> GSHMMSNANPYENNNPYAENYEMQEDLNNAPTGHYEGSDDFVAFMNKINSINANLSRYENIINQIDAQHKDLLTQVSEEQEMELRRSLDDYISQATDLQYQLKADIKDAQRDGLHDSN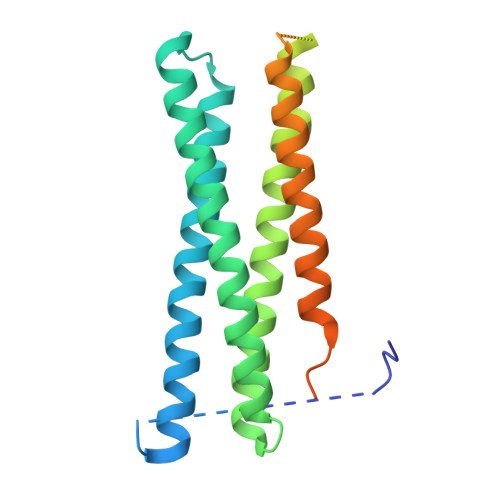KQAQAENCRQKFLKLIQDYRIIDSNYKEESKEQAKRQYTIIQPEATDEEVEAAINDVNGQQIFSQALLNANRRGEAKTALAEVQARHQELLKLEKTMAELTQLFNDMEELVIEQQENVDVIDKNVEDAQQDVEQGVGHTNKAVKSARKARKNKIRC> MQALRRGAAIPSRLLPRRDSWMSLAPFVAPNNAAAWRKLRDGAQEVQTVIERQSTPGKPQQIDWAKWESQIAHKDILNCLKTFYTNQVQILDRALGALETAKTPAPCEGAEKGWALFDAALSACAKSVEKSEELLSNGARALWVSCSNPPVWKVNTNEWLDSDQ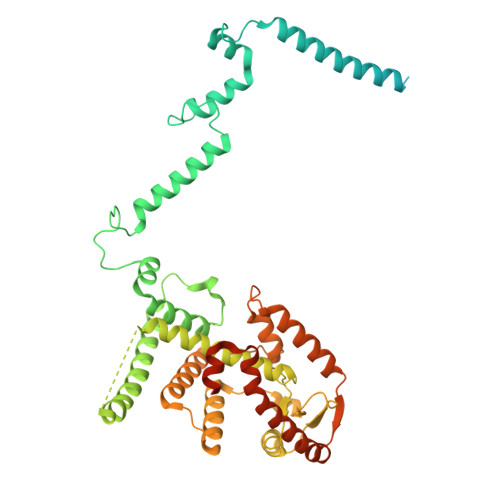YWQAFVEKHHFYSQYQPGVVDPEAPQEVEAFKQAWHSRMGKFNDRSDTPMLYAYMNELPSWEYYDLHRSAFLEHMTYFLVRTGGDFRFFPEMPPWQWLAHMENLRFKLLSVAQSRRSQLQLANLERERALDFLPVDVEHHGEEYTQKFLQYETELFQACAARLMGHFMFLCDPFIPVQSAEALSAVTRVDNGKGKLFSLGDDVNALFYLPEQQRRDVERPTQAVQTLLGHLEATGRPFNPCYSELLHVHAEVLEERGEHWLTAPGECVSQAFLRRLRTDDPAYEVYCSYFKEMYERFAGAKEVSMEDGRKRLATIEKNAQEEAAAYGLALKTMGSAELAHKAREGAAKLEQLRKAQEKAAGKSAQTVQENKM>MVRRQAPSAYIVLDPGHGGQDPGAVAPDGTREADLNLAQALTLKEYLVALGYRVGFTRTSDVYVPLSERIAMARRMGARLFISVHHDTPTASRPGVYYSPHPGSEELARTVAAALGEGAWVRPSSASRFGRLYIDDFPGPAILVEFGPTRPISRAERIARAQAVASPIAEFARRWT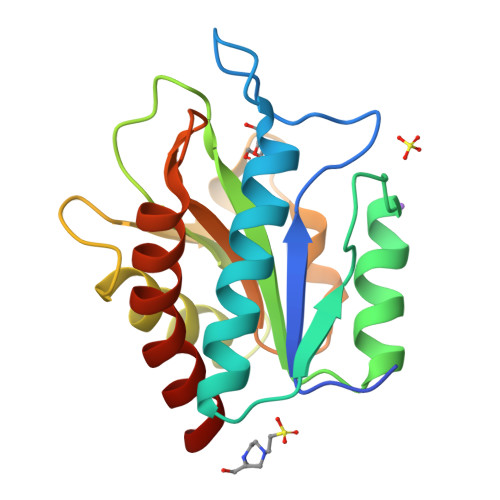A[5x]> ASMTGG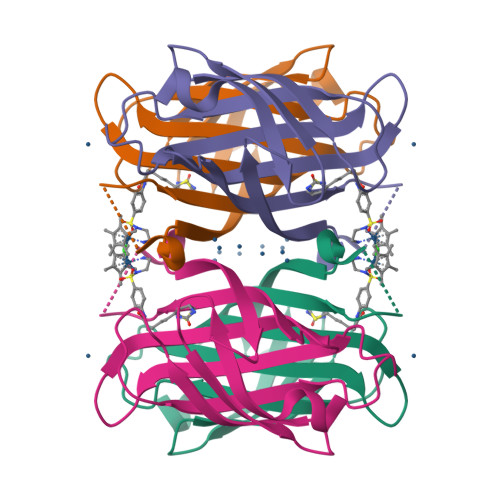QQMGRDQAGITGTWYNQLGSTFIVTAGADGALTGTYESAVGNAESRYVLTGRYDSAPATDGSGTALGWTVAWKNNYRNAHSATTWSGQYVGGAEARINTQWLLTVGTTSPLSEALTKANSPAEAYKASRGAGANAWASTLVGHDTFTKVKPSAASIDAAKKAGVNNGNPLDAVQQ4-(pyrrolidin-1-yl)-1-{4-[2-(pyrrolidin-1-yl)ethyl]phenyl}piperidine | C21 H33 N3 | 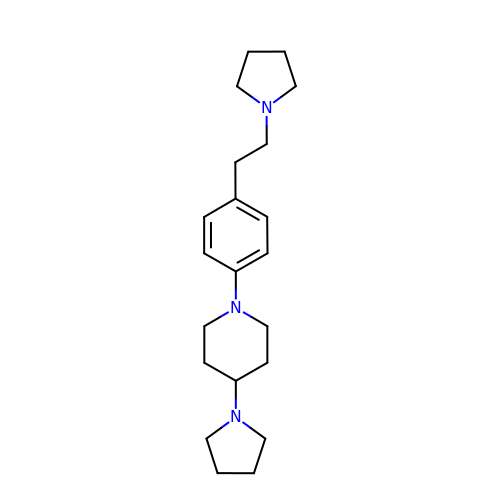JPTZZWFKOIEDMU-UHFFFAOYSA-N>MRKAIIVGVGMTPVGE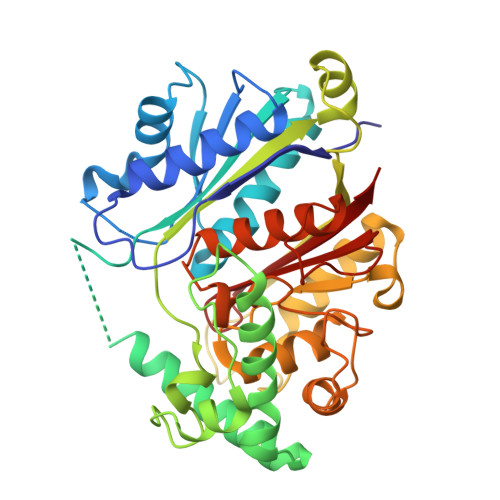HWRSSLRDLAVEAILNAMDDAGIDKVDSLYVGNMASGSFVEQENLGALIADWAGLGNIPAVKIEAACASGGAAVQEGAKAVLSGLEDVVLVVGVEKMTDAWPSDATRYLGYAADAEWELFHGASFVALNALIMRLYMNTYGYKEEDLALFAVNAHANGAKNPYAMFKKPITVETVMKSPYIADPLKLFDASPVCDGAAAVIITTPEKAKELGIPKDKWIEIAGMGRAIDTINLANREDFLTLKAATIAAERAYKMAGVKPEDVDFFEVHDAFTVMAALSLEALGVAKKGEGAKLAIEGQIAIDGDYPIQTMGGLKARGHPVGATGVYQVVEAVLQLRGEAPDGIQVPDAEVGLTQNIGGTGSNITVTVLRRV[3x]>[47x]MRITFNDVKTSLGITESYDIVNAIRNSQGDNFKSYVPLATANNVAE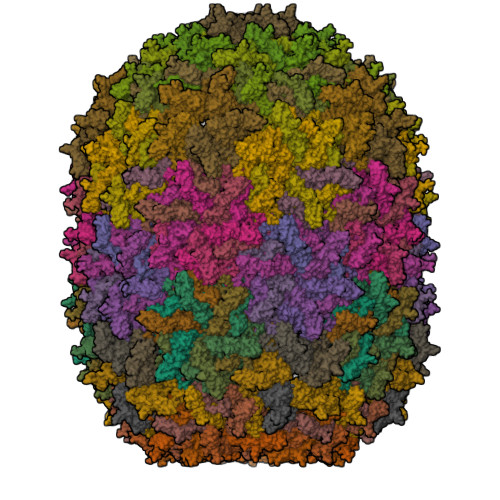VGAGILINQTVQNDFITSLVDRIGLVVIRQVSLNNPLKKFKKGQIPLGRTIEEIYTDITKEKQYDAEEAEQKVFEREMPNVKTLFHERNRQGFYHQTIQDDSLKTAFVSWGNFESFVSSIINAIYNSAEVDEYEYMKLLVDNYYSKGLFTTVKIDEPTSSTGALTEFVKKMRATARKLTLPQGSRDWNSMAVRTRSYMEDLHLIIDADLEAELDVDVLAKAFNMNRTDFLGNVTVIDGFASTGLEAVLVDKDWFMVYDNLHKMETVRNPRGLYWNYYYHVWQTLSVSRFANAVAFVSGDVPAVTQVIVSPNIAAVKQGGQQQFTAYVRATNAKDHKVVWSVEGGSTGTAITGDGLLSVSGNEDNQLTVKATVDIGTEDKPKLVVGEAVVSIRPNNASGGAQA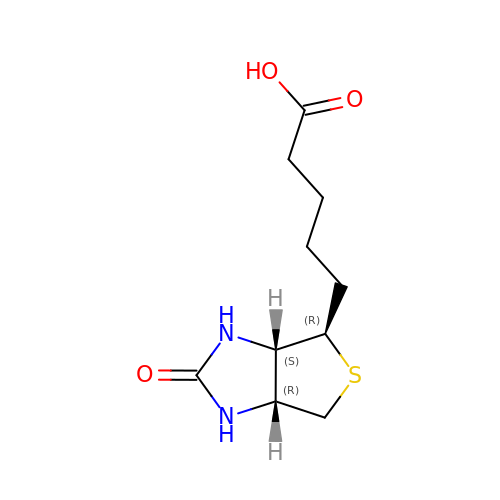EPI-BIOTIN | C10 H16 N2 O3 S | YBJHBAHKTGYVGT-OOZYFLPDSA-N> EFRHDSRKIPKVGHTFFQKPESCPPVPGGSMKLDIGIINENQRVSMSRNIESRSTSPWNYTVTWDPNRYPSEVVQAQCRNLGCINAQGKEDISMNSVPIQ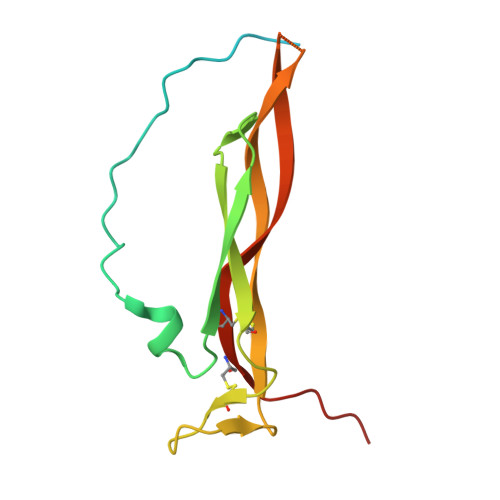QETLVVRRKHQGCSVSFQLEKVLVTVGCTCVTPVIHHVQ> TRGTRRIITGE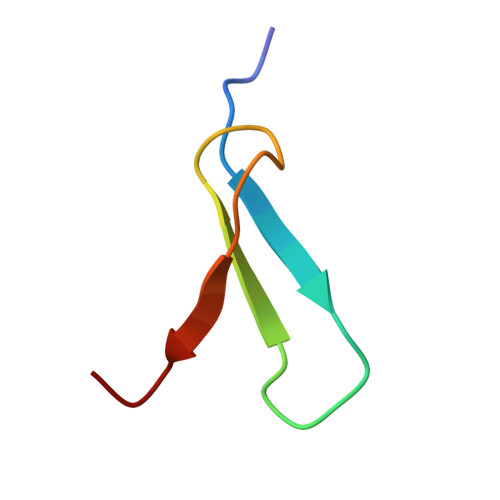ATQEDYYTGDHYATFSLIDKTC> MANPYERGPNPTDALLEARSGPFSVSEENVSRLSASGFGGGTIYYPRENNTYGAVAISPGYTGTEASIAWLGERIASHGFVVITIDTITTLDQPDSRAEQLNAALNHMINRASSTVRSRIDSSRLAVMGHSMGGGGSLRLASQRPDLKAAIPLTPWHLNKNWSSVRVPTLIIGADLDTIAPVLTHARPFYNSLPTSISKAYLELDGATHFAPNIPNKIIGKYSVAWLKRFVDNDTRYT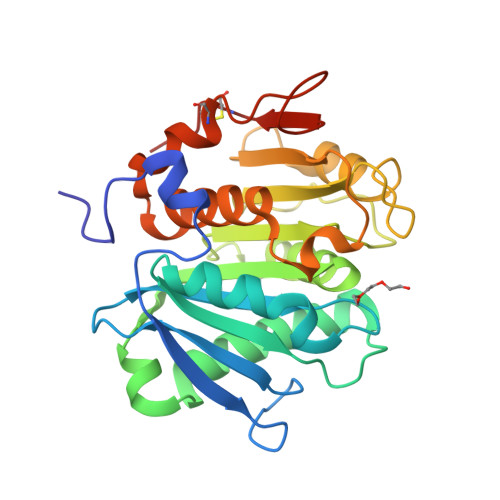QFLCPGPRDGLFGEVEEYRSTCPFLEHHHHHH6-methyl-2-oxidanylidene-chromene-3-carboxylic 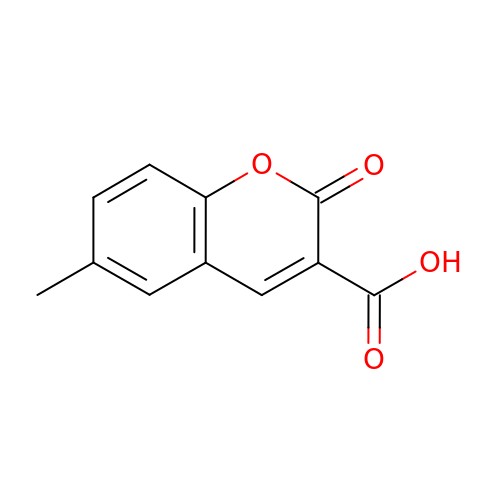acid | C11 H8 O4 | FJICLQQBBFWGMZ-UHFFFAOYSA-N>MSKRILFIVGSFSEGSFNRQLAKKAETIIGDRAQVSYLSYDRVPFFNQDLETSVHPEVAHAREEVQEADAIWIFSPVYNYAIPGPVKNLLDWLSRSLDLSDPTGPSVLQDKIVTVSSVANGASPEEVFEDYRSLLPFIRMHLVDQLTGVPINSEAWSTGILKVSAEKL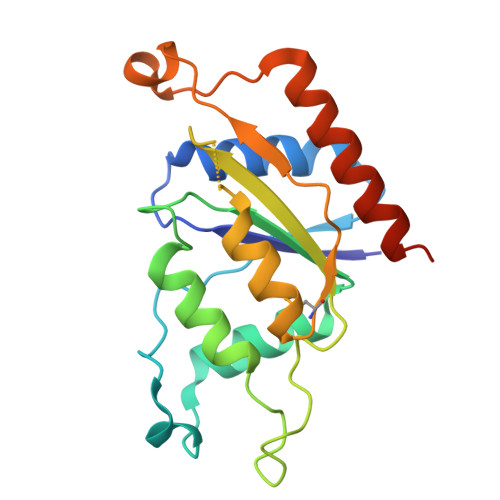AELSAQADALLSAIENLEHHHHHH[2x]>[2x]TTPSMEDYIEQIYMLIEEKGYARVSDIAEALAVHPSSVTKMVQKLDKDEYLIYEKYRGLVLTSKGKKIGKRLVYR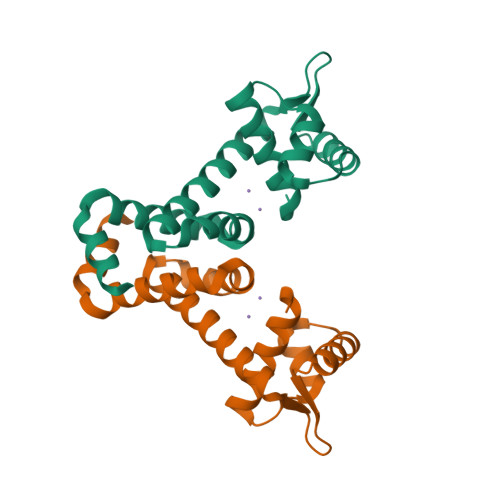AELLEQFLRIIGVDEEKIYNDVEGIEHHLSWNSIDRIGDLVQYFEEDDARKKDLKSIQKKTEHHNQ> SVVDTVAILKGLRDRYEAHHRINISDEAIEAAVKLSNRYVSDRFLPDKAIDLIDEASSKVRLKSHTTPNNLKEIEQEIEKVKNEKDAAVHAQEFENAANLRDKQTKLEKQYEEAKNEWKNAQNG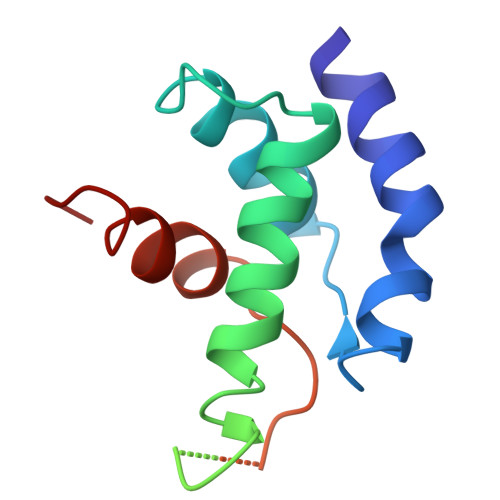MSTSLSEEDIAEVIAGWTGIP One such enzyme is 2-hydroxyacyl-CoA lyase/synthase (HACL/S), which catalyzes the reversible cleavage of 2-hydroxyacyl-CoA (2hcCoA) into formyl-CoA (fCoA) and an aldehyde or ketone. Originally identified in the mammalian α-oxidation pathway of 3-methyl-branched fatty acids, HACL/S has demonstrated remarkable catalytic reversibility, as it is capable of condensing fCoA with various substrates covering a wide range of aldehydes and ketones with different carbon chain lengths. All the enzymes are tetramers, specifically dimers of dimers (α2), where α2 dimer represents a catalytical unit. The three domains have specific functions: the N-terminal domain binds the pyrimidine of ThDP (PYR), the middle domain has a regulatory function (R) and binds ADP, and the C-terminal domain binds the pyrophosphoryl group (PP) of ThDP.

We have determined ten high-resolution structures of enzymes from the HACL/S sub-family, including DhcHACL/S, CcHACL/S, TbHACL/S, CfhHACL/S, and ApbHACL/S and measure kinetic parameters for all purified enzymes. All structures contain well-defined bound ThDP and ADP. All our HACL/S structures contain bound ADP in the R domain, which assumes the Rossmann fold nucleotide binding unit.

>[2x]MPEGPVAEIDGQTIIARALKQQGVEAMFGVVGIPVTGIAAAAQREGIKYVGMRHEMPATYAAQAVSYLGGRLGTALAVSGPGVLNAVAAFANAWSNRWPMILIGGSYEQTGHLMGFFQEADQLSALKPYAKYAERVERLERIPIYVAEAVKKALHGVPGPAYLELPGDIITAKIDESKVEWAPRVPDPKRTLSDPADVEAAIAALKTAQQPLIIVGKGVAASRAEVEIRAFVEKTGIPYLAMPMAKGLIPDDHDQSAAAARSFVLQNADLIFLVGARLNWMLHFGLPPRFRPDVRVVQLDFNPEEIGINVPTEVGMIGDAKATLSQLLDVLDRDGWRFPDDSEWVTAVSAEARQNAEAVQAMMQEDTQPLGYYRALRSIDERLPKDAIFVAEGASTMDISRTVINQYLPRTRLDAGSFGSMGLGHGFAIGAATQFPGKRVICLQGDGAFGFAGTECEVAVRYNLPITWIVFNNGGIGGHRAELFERDQKPVGGMSLGARYDILMQGLGGAAFNATNSDELDAAIEAALKIDGPSLINVPLDPDAKRKPQKFGWLTRTNE>ATGDEWWAKCKQVDVLDSEMSYYDSDPGKHKNTVIFLHGNPTSSYLWRNVIPHVEPLARCLAPDLIGMGKSGKLPNHSYRFVDHYRYLSAWFDSVNLPEKVTIVCHDWGSGLGFHWCNEHRDRVKGIVHMESVVSPLKGWESFPETARDIFQALRSEAGEEMVLKKNFFIERLLPSSIMRKLSEEEMDAYREPFVEPGESRRPTLTWPREIPIKGDGPEDVIEIVKSYNKWLSTSKDIPKLFINADPG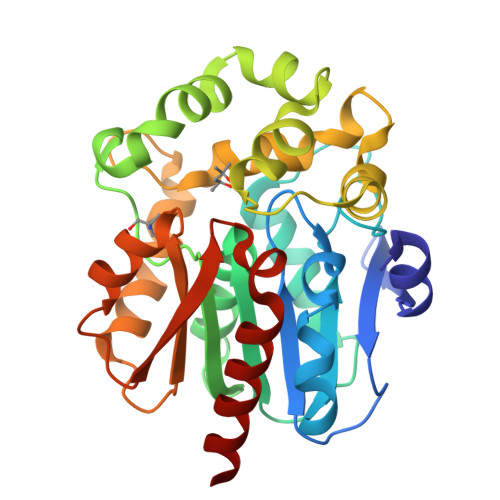FFSNAIKKVTKNWPNQKTVTVKGLHFLQEDSPEEIGEAIADFLNELTK[2x]>[2x]MALLTPIPSPMVNLTQVIDPTEQLAYFPKITFERLKNYDTSSNYAKGKLTRNYMILLPWQHVNRYNFVFSSTGCKVSLKTCIGKLMKDLNPKVLYFIGEGAG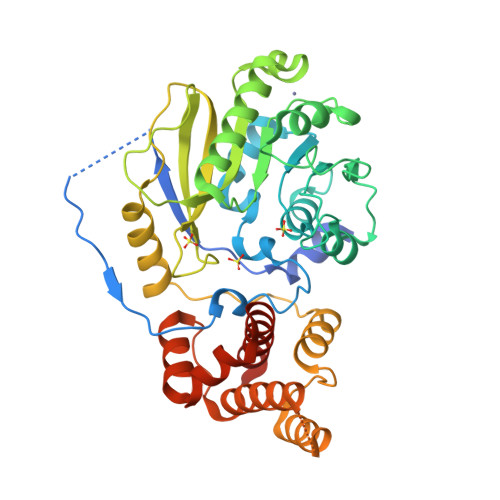NWMARTACEYPDIKFVYRSLKDDLDHHYPLEYQRVIGELSRIIDSGEGLSMETTDATQKTHWDLIHRVSKDALLITLCDAEFKDRDDFFKMVILWRKHVLSCRICTTYGTDLYLFAKYHAKDCNVKLPFFVRSVATFIMQGSKLSGSECYILLTLGHHNNLPCHGEIQNSKMKIAVCNDFYAAKKLDNKSIEANCKSLLSGLRIPINKKELNRQRRLLTLQSNHSSVATVGGSKVIESKWLTNKANTIIDWLEHILNSPKGELNYDFFEALENTYPNMIKLIDNLGNAEIKKLIKVTGYMLVSKKSGHHHHHH> MAAPNRDPPGYRYAAAMVPTGSLLSTIEVASHRRLFDFFSRVRSDANSLYDVEFDALLGSYCNTLSLVRFLELGLSVACVCTKFPELAYMNEGRVQFEVHQPLIARDGPHPIEQPTHNYMTKIIDRRALNAAFSLATEAIALLTGEALDGTGIGAHRQLRAIQQLARNVQAVLGAFERGTADQMLHVLLEKAPPLALLLPMQRYLDNGRLATRVARATLVAELKRSFCETSFFLGKAGHRREAVEAWLVDLTTATQPSVAVPRLTHADTRGRPVDGVLVTTAPIKQRLLQSFLKVEDTEADVPVTYGEMVLNGANLVTALVMGKAVRSLDDVGRHLLEMQEEQLDLNRQTLDELESAPQTTRVRADLVSIGEKLVFLEALEKRIYAATNVPYPLVGAMDLTFVLPLGLFNPVMERFAAHAGDLVPAPGHPDPRAFPPRQLFFWGKDRQVLRLSLEHAIGTVCHPSLMNVDAAVGGLNRDPVEAANPYGAYVAAPAGPAADMQQLFLNAWGQRLAHGRVRWVAEGQMTPEQFMQPDNANLALELHPAFDFFVGVADVELPGGDVPPAGPGEIQATWRVVNGNLPLALCPAAFRDARGLELGVGRHAMAPATIAAVRGAFDDRNYPAVFYLLQAAIHGSEHVFCALARLVVQCITSYWNNTRCAAFVNDYSLVSYVVTYLGGDLPEECMAVYRDLVAHVEALAQLVDDFTLTGPELGGQAQAELNHLMRDPALLPPLVWDCDALMRRAALDRHRDCRVSAGGHDPVYAAACNVATADFNRNDGQLLHNTQARAADAADDRPHRGADWTVHHKIYYYVMVPAFSRGRCCTAG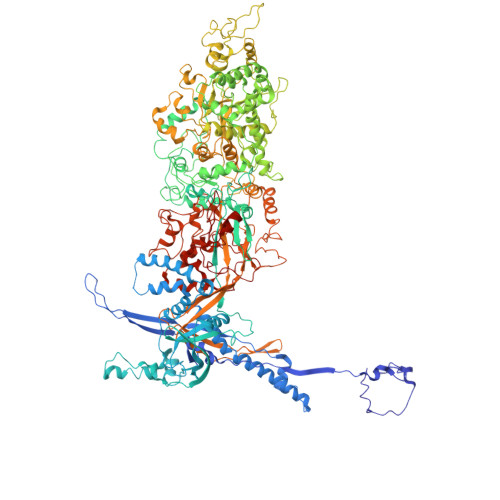VRFDRVYATLQNMVVPEIAPGEECPSDPVTDPAHPLHPANLVANTVNAMFHNGRVVVDGPAMLTLQVLAHNMAERTTALLCSAAPDAGANTASTTNMRIFDGALHAGILLMAPQHLDHTIQNGDYFYPLPVHALFAGADHVANAPNFPPALRDLSRQVPLVPPALGANYFSSIRQPVVQHVRESAAGENALTYALMAGYFKISPVALHHQLKTGLHPGFGFTVVRQDRFVTENVLFSERASEAYFLGQLQVARHETGGGVNFTLTQPRGNVDLGVGYTAVVATATVRNPVTDMGNLPQNFYLGRGAPPLLDNAAAVYLRNAVVAGNRLGPAQPVPVFGCAQVPRRAGMDHGQDAVCEFIATPVSTDVNYFRRPCNPRGRAAGGVYAGDKEGDVTALMYDHGQSDPSRAFAATANPWASQRFSYGDLLYNGAYHLNGASPVLSPCFKFFTSADIAAKHRCLERLIVETGSAVSTATAASDVQFKRPPGCRELVEDPCGLFQEAYPLTCASDPALLRSARNGEAHARETHFAQYLVYDASPLKGLAL4-[2,2-bis(hydroxymethyl)-5-oxopyrrolidin-1-yl]-3-[(dipropylamino)methyl]benzoic acid | C20 H30 N2 O5 | 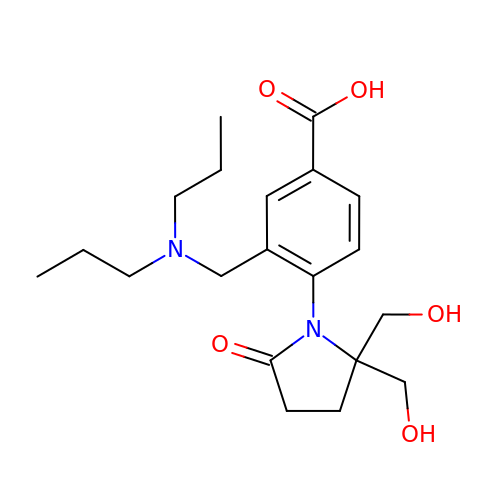IYODICUSAICAQL-UHFFFAOYSA-N> MDLSELERDNTGRCRLSSPVPAVCLKEPCVLGVDEAGRGPVLGPMVYAICYCPLSRLADLEALKVADSKTLTENERERLFAKMEEDGDFVGWALDVLSPNLISTSMLGRVKYNLNSLSHDTAAGLIQYALDQNVNVTQVFVDTVGMPETYQARLQQHFPGIEVTVKAKADSLFPVVSAASIFAKVARDKAVKNWQFVENLQDLDSDYGSGYPNDPKTKAWLRKHVDPVFGFPQFVRFSWSTAQAILEKEAEDVIWEDSEAEEDPERPGKITSYFSQGPQTCRPQAPHRYFQERGLEAASSL;> MGSSHHHHHHSQDPNSLEVLFQGPMAGGRDRGDLAARQLVFLLPEHLKDASKKKKKSSLLFVKLANPHSGEGATYLIDMCLQQLFEIKVFKEKHHSWFINQSVQSGGLLHFATPMDPLFLLLHYLLKAGKEGKYQPLDQVVVDDTFPDCTLLLRFPELEKSLRHVTEEKEVNSKKYYKYSSEKTLKWLEKKVNQTVVALKANNVNVGARVQSSAYFSGGQVSRDKEEDYVRYAHGLISDYIPKELSDDLSKFLKLPEPPASLTNPPSKKLKLSDEPVEAKEDYTKF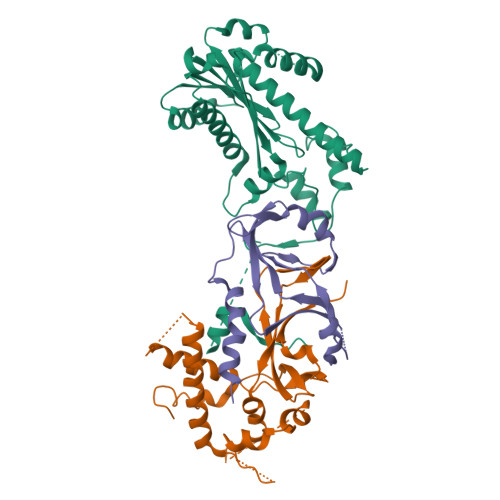NTKDLKTGKKNSKMTAAQKALAKVDKSGMKSIDAFFGAKNKKTGKI;> MKNPEEAADGKQRIHLRPGSLRGAAPAKLHLLPCDVLVSRPAPVDRFFTPAVRHDADGLQASFRGRGLRGEEVAVPPGFAGFVMVTEEKGEGLIGKLNFSGDAEDKADEAQEPLERDFDRLIGATGSFSHFTLWGLETVPGPDAKVHRALGWPSLAAAIHAQVPED>[5x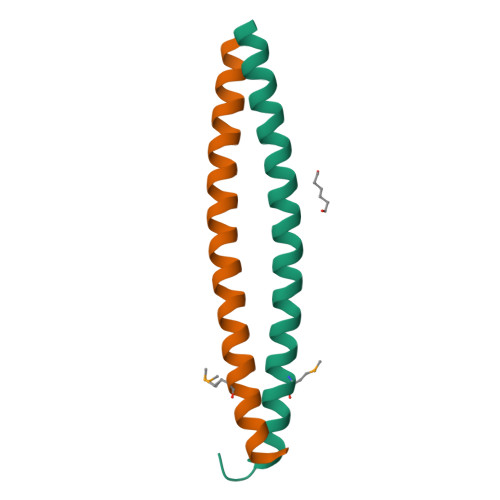]MRGSHHHHHHGMASIEGRGSLRDLQYALQEKIEELRQRDALIDELELELDQKDELIQMLQNELDKYRSVIRP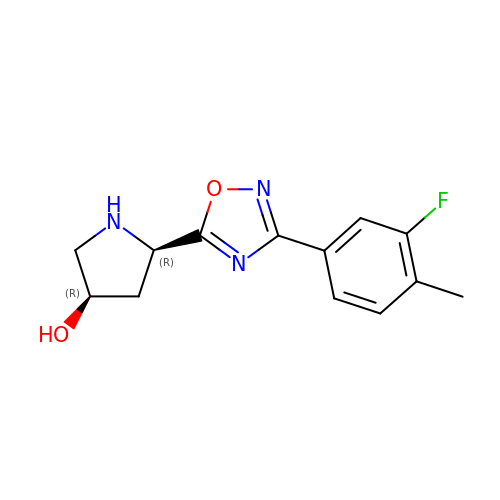(3R,5R)-5-[3-(3-fluoro-4-methylphenyl)-1,2,4-oxadiazol-5-yl]pyrrolidin-3-ol | C13 H14 F N3 O2 | UGTHZDBHYCLBLY-MWLCHTKSSA-N(3S,6E)-3,7,11-trimethyldodeca-6,10-dien-1-yl 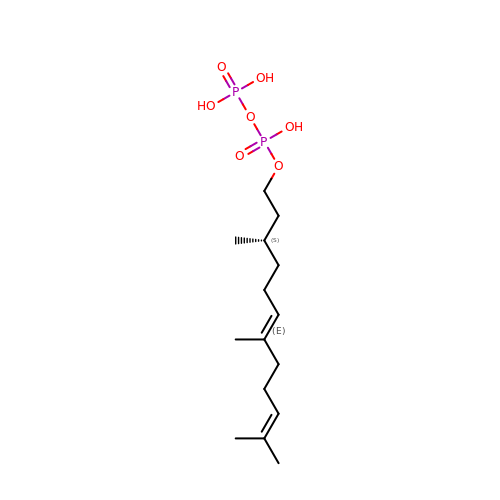trihydrogen diphosphate | C15 H30 O7 P2 | UGQVBUXMCRXOIF-HNRFISLBSA-N> MREWLDILGNGLLRKKTLVPGPPGSSRPVKGQVVTVHLQTSLENGTRVQEEPELVFTLGDCDVIQALDLSVPLMDVGETAMVTADSKYCYGPQGRSPYIPPHAA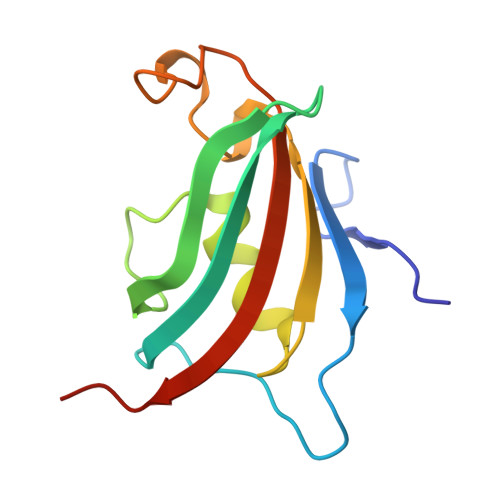LCLEVTLKTAVDGPDLE> MVFYSFVLVMKPRQRRFTSQALREIGVAVYSNGGLIRSITNEGIMRPYSRFRDADNTPLTYARYIILQLDMGEEE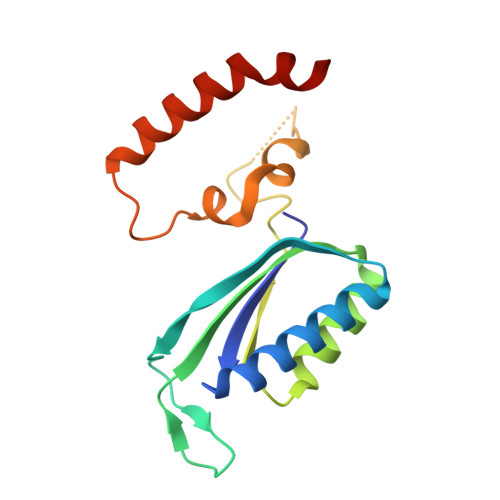MGKVDKIIREHQDVLMALKLNNLERPVGIRSGNKELQAAYFPLDTFTRLEEEINWSPQTSADIYTQLEMNWKEFSRTRWSSFLRN>MGLEKTVKEKLSFEGVGIHTGEYSKLIIHPEKEGTGIRFFKNGVYIPARHEFVVHTNHSTDLGFKGQRIKTVEHILSVLHLLEITNVTIEVIGNEIPILDGSGWEFYEAIRKNILNQNREIDYFVVEEPIIVEDEGRLIKAEPSDTLEVTYEGEFKNFLGRQKFTFVEGNEEEIVLARTFCFDWEIEHIKKVGLGKGGSLKNTLVLGKDKVYNP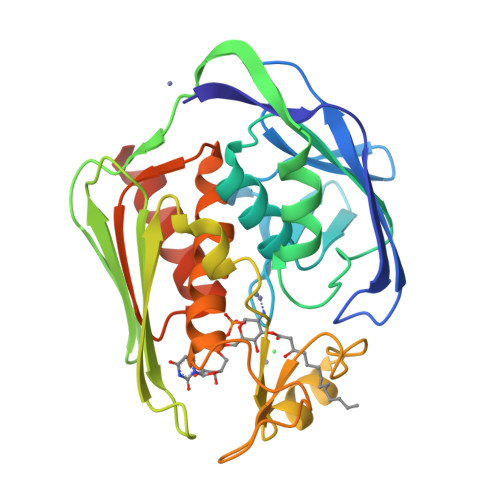EGLRYENEPVRHKVFDLIGDLYLLGSPVKGKFYSFRGGHSLNVKLVKELAKKQKLTRDLPHLPSVQAL[2x]> NGIVPDAGHQGPDVSAVNGGTQVINIVTPNNEGISHNQYQDFNVGKPGAVFNNALEAGQSQLAGHLNANSNLNGQAASLILNEVVSRNPSFLLGQSEVFGIAAEYVLSNPNGITCDGCGFINTSRSSLVVGNPLFENGQLKGYSTLNNTNLLSL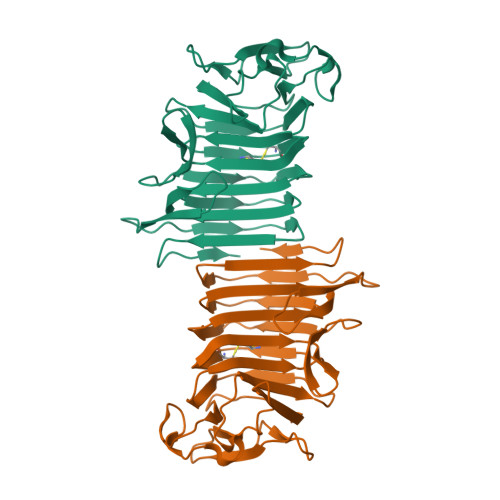GKNGLNTTGLLDLIAPRIDSRGKITAAEISAFTGQNTFSQHFDILSSQKPVSALDSYFFGSMQSGRIRIINTAEGSGVKLAGHHHHHH(2-{2-[(2S)-3-methylbutan-2-yl]-5-phenyl-1H-indol-3-yl}ethane-1,1-diyl)bis(phosphonic 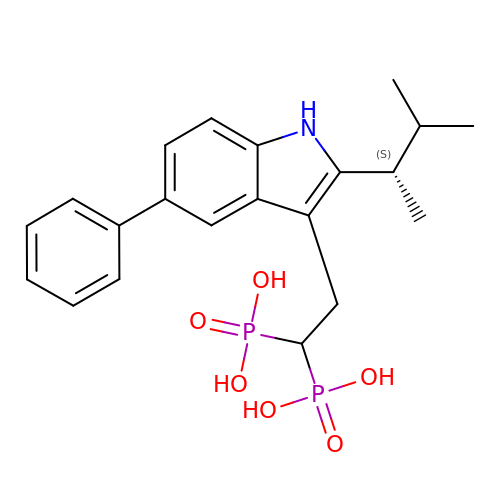acid) | C21 H27 N O6 P2 | PCZFJEHMSDBRJQ-AWEZNQCLSA-N5-cyclohexylspiro[1H-indole-3,4'-oxane]-2-one | C18 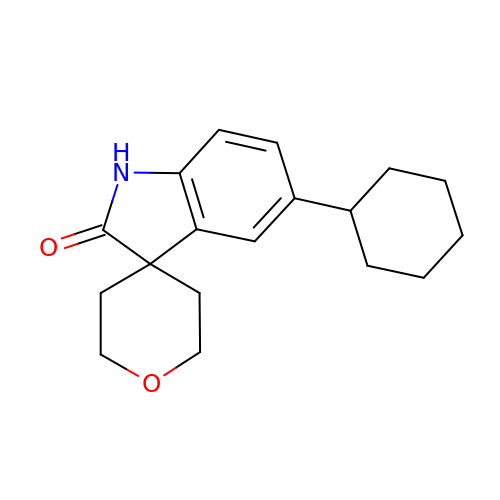H23 N O2 | RZFQOJSXHMJDFD-UHFFFAOYSA-N>MFERIDYYAGDPILGLVEKFAADNNPDKVNLGIGIYYDESGVMPVLDCVKIAEQRIADPISPRPYLPMAGLPGHRKGCQELLFGKDAPVLKDGLVATIATIGGSGALKVGAEFIHEWFPQSKCYVSDPTWGNHIAIFEGCDIEVGKYPYYDTATGGIKFDEMIAFFETLNKDDVLLLHPCCHNPTGVDLTREQWDTVLNVIQERELIPFMDIAYQGFGEDMDSDAYAIRKAVDMGLPLFVSNSFSKNLSLYGERVGGLSVVCPTVDETERVFGQLNSTVRRIYSSPPSHGGRVVDIVMNDAALHEQWVGEVYAMRDRIKSMRTKLKSVLEAKISGRNFDYLTAQNGMFSFTGLTPEQVERLQSEFGIYMISNSRMCVAGLNSSNIDYVANAMVDVLKD[2x]

The psychrophilic aromatic aminotransferase from Psychrobacter sp. B6 is a representative of pyridoxal phosphate (PLP)-dependent enzymes. PsyArAT exhibits an activity typical for ArAT: transamination, which is a transfer of an amine group between aromatic α-amino acids and α-ketoacids. The mechanism of active site adjustment toward substrates of psychrophilic aromatic amino acid aminotransferase (PsyArAT) from Psychrobacter sp. B6 is discussed based on crystal structures of complexes with four hydroxy-analogs of substrates: phenylalanine, tyrosine, tryptophan and aspartic acid. These competitive inhibitors are bound in the active center of PsyArAT but do not undergo transamination reaction, which makes them an outstanding tool for examination of the enzyme catalytic center.

The hydrogen bonds network made by a FOH ligand were slightly different for both monomers of the PsyArAT/FOH complex. In either case, carboxyl group of FOH creates two parallel hydrogen bonds with the guanidine group of Arg374 (3.2 Å and 3.0 Å in monomer A, 2.3 Å and 2.8 Å in monomer B), one with a side-chain nitrogen of Asn183 (3.2 Å for both monomers) and one with an indole ring nitrogen of Trp130 (3.4 Å for both pockets). Interactions between the ligand carboxyl group and the cofactor was present only in pocket B, where it had contact with formyl oxygen (3.1 Å). The interaction with the peptide bond nitrogen of Gly34 was made by the carboxyl oxygen of FOH (2.8 Å) in the active site of pocket B, while the ligand in the neighboring subunit made contact with the same residue, using its hydroxyl group (3.4 Å). Generally, most of the differences were a result of different placement of the -OH group in the pockets due to a rotation of ligand by 90°. Thus, in monomer A, besides the aforementioned interaction with Gly34, the hydroxyl group of FOH made bonds with the carbonyl oxygen of Gly34 (3.4 Å), the hydroxyl oxygen of Tyr214 (3.3 Å) and PLI Schiff base nitrogen (3.5 Å). In pocket B, the -OH of the ligand made the second contact with Trp130 (3.3 Å) and created two hydrogen bonds with a PLP molecule, first with the aldehyde group (2.3 Å) and the second with the hydroxyl oxygen of the cofactor (3.1 Å). In the catalytic center of both complexes, the Arg280* switch was in the “down” position; however, in the case of PsyArAT/YOH, it was placed a little deeper than in the PsyArAT/FOH complex. As stated, in PsyArAT/FOH complex, Arg280* was placed slightly further from the ligand; in the active site of monomer A, it interacted with Asp11 (2.8 Å) like in the previous case, but it also reached Tyr8 hydroxyl oxygen (3.2 Å). In the active pocket of monomer B, Arg280* made an even shorter bond with the OH group of Tyr8 (2.8 Å), but the interaction with Asn132 (2.9 Å) replaced the one with Asp11.>[2x]MAHHHHHHMSVEVEYLQHEDYLYRTSKLKEIRDLGINPYPYQYTDCLEVQEIRNQFVDNELGDSEAAFRKETPKVRFAGRLVLFRSMGKNAFGQILDNDAKIQVMFNRDFSAVAGLAADAGISPIKFIEKKLDLGDILGLEGYLFFTHSGELTVLVETVTLLCKSLISLPDKHAGLADKEIRYRKRWADLISSEDVRKTFLTRSRILKLIREYMDQQSFLEVETPILQTVYGGAEATPFVTTLQALHAEMFLRISLEIALKKLLVGGMSRVYEIGKVFRNEGIDRTHNPEFT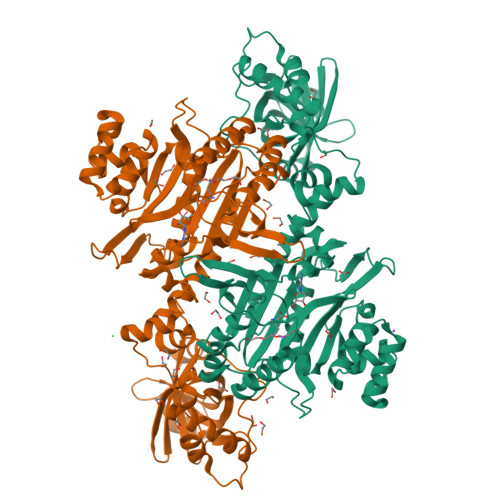MIEAYAAYWDYNDVMKCVENLVEYIVRALNNGETQVQYSHLKSGPQVVDFKAPWIRMTMKESISVYGGVDVDLHADHELRKILETQTSLPEKTYVHASRGELIALLFDELVCDKLIAPHHITDHPLETTPLCKTLRSGDETLVERFESFCLGKELCNAYSELNDPLQQRKLLEEQMRKKALNPDSEYHPIDEEFLEALCQGMPPAGGFGIGIDRLVMMLTDAASIRDVLFFPVMRRIEAKKD>[2x]PYIEIFEQPRQRGMRFRYKCEGRSAGSIPGEHSTDNNKTFPSIQILNYFGKVKIRTTLVTKNEPYK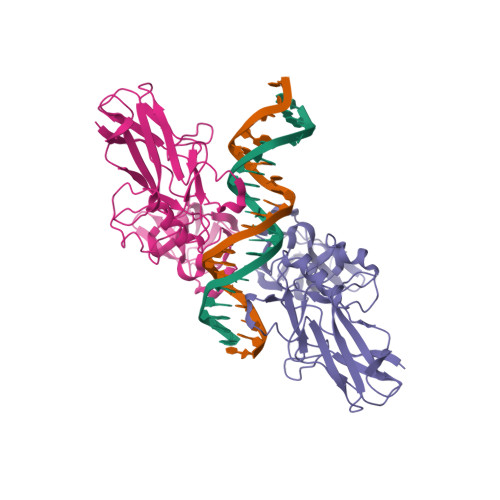PHPHDLVGKDCRDGYYEAEFGPERRVLSFQNLGIQCVKKKDLKESISLRISKKINPFNVPEEQLHNIDEYDLNVVRLCFQAFLPDEHGNYTLALPPLISNPIYDNRAPNTAELRICRVNKNCGSVKGGDEIFILCDKVQKDDIEVRFVLDNWEAKGSFSQADVHRQVAIVFRTPPFLRDITEPITVKMQLRRPSDQEVSEPMDFRYLPD> NNYVYIDPTQLPYDHKWEFPRNRLSFGKTLGAGAFGKVVEATAYGLIKSDAAMTVAVKMLKPSAHLTEREALMSELKVLSYLGNHMNIVNLLGACTIGGPTLVITEYCCYGDLLNFLRRKRDSFICSKTSPAIMEDDELALDLEDLLSFSYQVAKGMAFLASKNCIHRDLAARNIL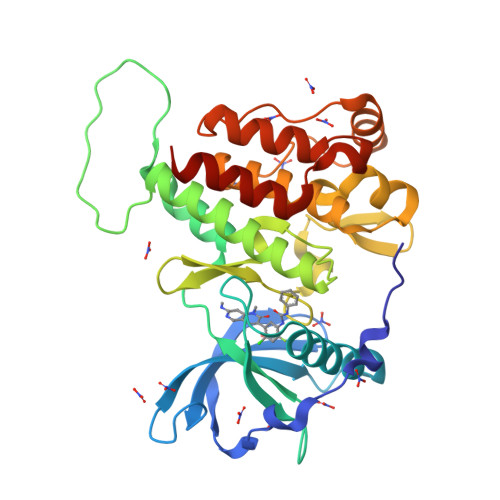LTHGRITKICDFGLARDIKNDSNYVVKGNARLPVKWMAPESIFNCVYTFESDVWSYGIFLWELFSLGSSPYPGMPVDSKFYKMIKEGFRMLSPEHAPAEMYDIMKTCWDADPLKRPTFKQIVQLIEKQISESTNHI> DAASDLKSRLDKVSSFHASFTQKVTDGSGAAVQEGQGDLWVKLPNLFNWHMTQPDESILVSDGKTLWFYNPFVEQATATWLKDATGNTPFMLIARNQSSDWQQYNIKQNGDDFVLTPKASNG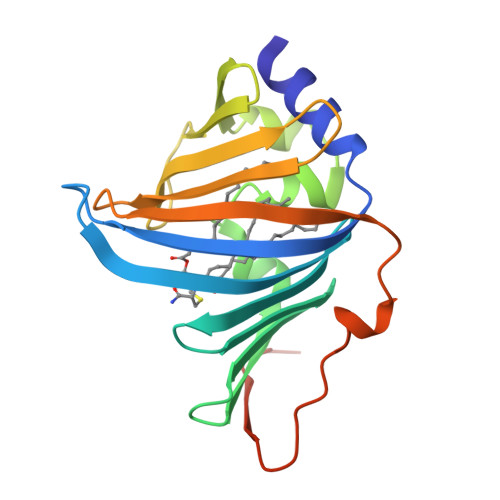NLKQFTINVGRDGTIHQFSAVEQDDQRSSYQLKSQQNGAVDAAKFTFTPPQGVTVDDQRKGSWSHPQFEK> GSVTHEQFKAA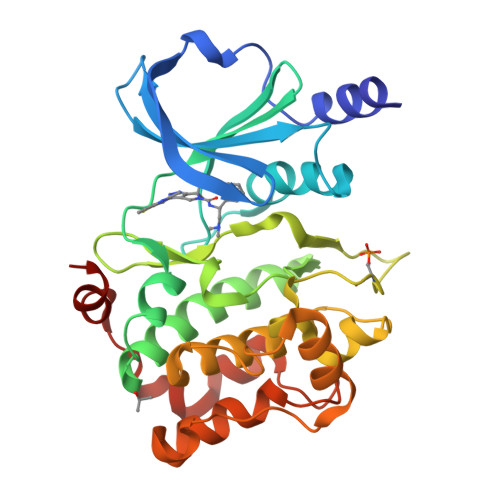LRMVVDQGDPRLLLDSYVKIGEGSTGIVCLAREKHSGRQVAVKMMDLRKQQRRELLFNEVVIMRDYQHFNVVEMYKSYLVGEELWVLMEFLQGGALTDIVSQVRLNEEQIATVCEAVLQALAYLHAQGVIHRDIKSDSILLTLDGRVKLSDFGFCAQISKDVPKRKSLVGTPYWMAPEVISRSLYATEVDIWSLGIMVIEMVDGEPPYFSDSPVQAMKRLRDSPPPKLKNSHKVSPVLRDFLERMLVRDPQERATAQELLDHPFLLQTGLPECLVPLIQLY CCs are quaternary structures comprising two or more α-helices supercoiled around each other with cyclic (Cn) or dihedral (Dn) symmetry. Here, we describe variants with all combinations of the aliphatic residues, Ile, Leu and Val, at a and d to give four classes of peptide: the ββ class, with a and d = Ile or Val; Lβ, a = Leu and d = Ile or Val; βL, a = Ile or Val and d = Leu; and LL, a = d = Leu. Peptides are named systematically appending the one-letter code for the amino acids at the a and d sites to “CC-Type2-“; e.g., CC-Hept becomes CC-Type2-LI. In summary, solution-phase data and X-ray crystal structures demonstrate conclusively that different classes of Type-2 coiled-coil (CC) peptides—i.e., based on abcdefg repeats with predominantly hydrophobic residues at a, d, e and g—adopt a range of distinct states.

Mutating Ile→Phe to give CC-Type2-LF rendered another collapsed structure, but with eight helices in two 21-symmetric 4-helix bundles interfaced by unusual bifurcated helices. Thus, the bulk of Phe cannot substitute for β-branching at d to maintain open α-helical barrels. Despite the complexity of these Phe-containing structures, they are CCs founded on KIH packing. Moreover, the KIH analysis revealed that helices with the same sequence participate in different quaternary arrangements. Similarly, the sequences with bulky Phe at a or d fit poorly to most structures other than their own.

>XGEFAQALKEFAKALKEFAWALKEFAQALKGX[8x]>[2x]MGRIKNKQFAVIGLGRFGGSICKELHRMGHEVLAVDINEEKVNAYASYATHAVIANATEENELLSLGIRNFEYVIVAIGANIQAS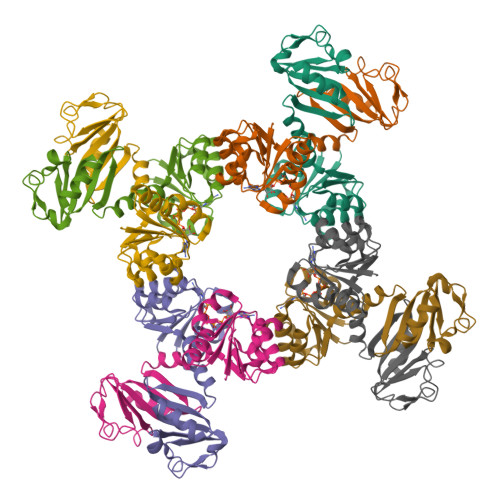TLTTLLLKELDIPNIWVKAQNYYHHKVLEKIGADRIIHPEKDMGVKIAQSLSDENVLNYIDLSDEYSIVELLATRKLDSKSIIDLNVRAKYGCTILAIKHHGDICLSPAPEDIIREQDCLVIMGHKKDIKRFENEGM>[2x]GIDPFTEEPTNLIKQKMDELIKHLNQKIVSLKREQQTISEECSANDRLGQDLFAKLAEKVRPSEASKFRTHVDAVGNITSLLLSLSERLAQTESSLETRQQER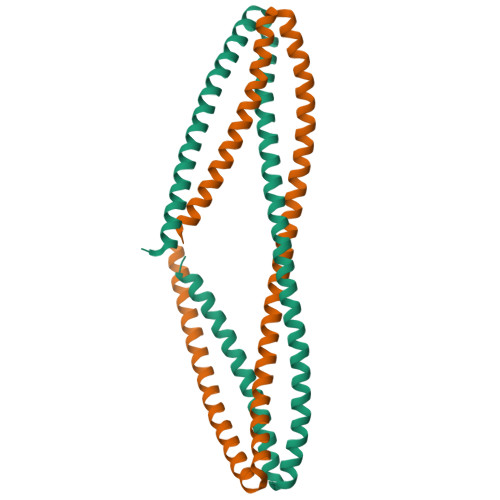GALESKRDLLYEQMEEAQRLKSDIERRGVSIAGLLAKNLSADMCADYDYFINMKAKLIADARDLAVRIKGSEEQLSSLSDALVQSDC>[2x]HMKIAVMTDSTSYLSQDLIDKYNIQIAPLSVTFDDGKNFTESNEIAIEEFYNKMASSQTIPTTSQPAIGEWITKYEMLRDQGYTDIIVICLSSGISGSYQSSYQAGEMVEGVNVHAFDSKLIAMIEGCYVLRAIEMVEEGYEPQQIIDDLTNMREHTGAYLIVDDLKNLQKSGRITGAQAWVGTLLKMKPVLKFEDGKIIPEEKVRTKKRAIQTLEKKVLDIVKDFEEVTLFVINGDHFEDGQALYKKLQDDCPSAYQVAYSEFGPVVAAHLGSGGLGLGYVGRKIRLT

Staphylococcus aureus FakB1 is a prototypical bacterial FA transfer protein that binds palmitate within a narrow, buried tunnel. Here, we use a combination of X-ray crystallography, NMR spectroscopy, MD simulations, site-directed mutagenesis, and functional biochemical assays to characterize the membrane-bound conformation of FakB. This study focuses on FakB1, an FA transfer protein from S. aureus that binds palmitic acid (16:0) before presenting it to FakA for phosphorylation and exchange with the membrane. The bacterial class of FA transfer proteins is called FakB, and the bound acyl chains are completely enclosed within the protein interior. The open conformation arises from a conformational change in the dynamic region that rotates helix α8 outward to uncover the FA-binding tunnel and reorganizes the adjacent α8-β9 loop into a new amphipathic helix.

The crystal structure of FakB1(A121I) was determined at 2.02 Å resolution. We observed two molecules (molA and molB) in different conformational states in the asymmetric unit. The prototypical FakB1 closed conformation was exemplified by molB, but in molA, the dynamic region undergoes a significant structural rearrangement. Specifically, Arg173 disengages from the FA and Ile94, helix α8 (Leu165 to Ser171) moves away from the protein, and residues 175 to 186 form a new α-helix that rotates away from the protein by ∼180° in concert with the movement of helix α8. Excluding the structural rearrangements observed in FakB1(A121I), the open and closed structures superimpose with an RMSD of 0.356 Å showing that the conformational change is confined to these residues. In FakB1(A121I), the bulkier side chain displaces the middle of the aliphatic chain of the FA by 0.9 Å and its distal end by ∼1.4 Å that, in turn, shifts the tunnel residues Val162, Leu191, and Leu271 and pushes against the dynamic region. In the open conformation, Arg173 becomes disengaged from FakB1, and the newly formed 12-residue helix that we designate as α8′ has a distinct exposed hydrophobic surface consisting of Ala177, Trp180, Val181, Leu184, and Leu185. We also note that the disengagement of Arg173 from the FA and the outward movements of α8 and α8′ disrupt the hydrogen bond network surrounding the FA carboxylate by breaking the key Ser171-His270 hydrogen bond and exposing His270 to solvent. The FakB1(A121I) is the highest-resolution crystal structure and was used as the representative open conformation for further analysis. Analysis of the open FakB1(A121I) crystal structure reveals a groove created by the conformational change that forms a channel extending from the FA-binding site to the electropositive end of the protein.>MHHHHHHSLLTEVETYVLSIVPSGPLKAEIAQRLEDVFAGKNTDLEVLMEWLKTRPILSPLTKGILGFVFTLTVPSERGLQRRRFVQNALNGNEDPNNMDKAVKLYSKLKSEITFHGAKEIALSYSAGALASCMGLIYNRMGAVTTEVAFGLVCATCEQIADSQHRSHRQM[2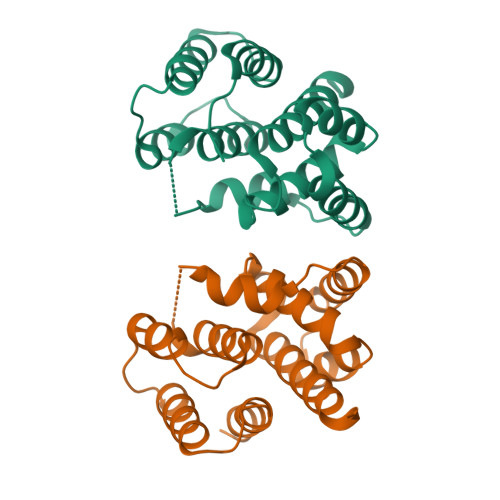x]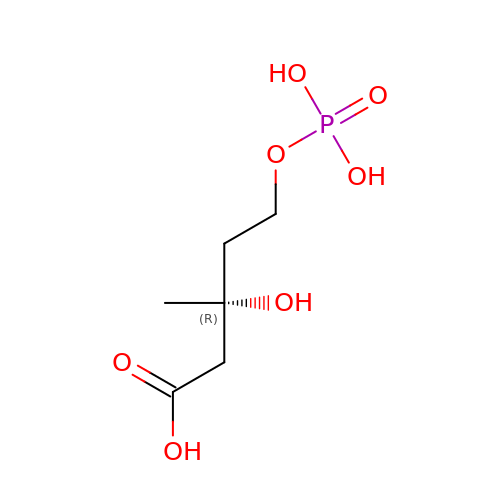(3R)-3-HYDROXY-3-METHYL-5-(PHOSPHONOOXY)PENTANOIC ACID | C6 H13 O7 P | OKZYCXHTTZZYSK-ZCFIWIBFSA-N>[2x]GPLGSSRVSVLS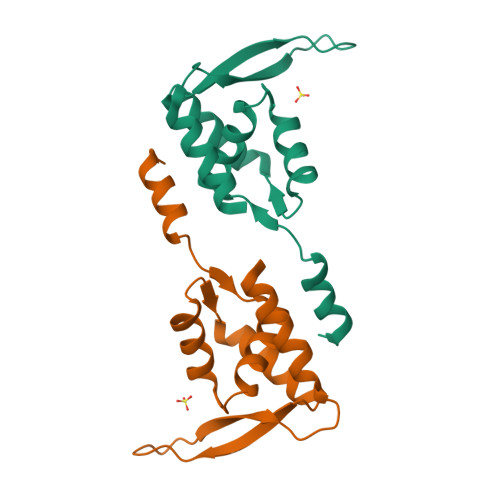MDFEDIYRFFQDPPPHYLSKELAVCYVLAVLRHEDSYGTELIQHLETHWPNYRLSDTVLYTALKFLEDEQIISGYWKKVEGRGRPRRMYQLAQANDDRSRDLAQLWERYLSSSAATDRQLIPVEAR> MSLRPLYMDVQATTPLDPRVLDAMLPYLINYYGNPHSRTHAYGWESEAAMERARQQVASLIGADPREIIFTSGATESNNIAIKGVARFYRSRKKHLITTQTEHKCVLDSCRSLEAEGFQVTYLPVQKSGIIDLKELEAAIQPDTSLVSVMTVNNEIGVKQPIAEIGRICSSRKVYFHTDAAQAVGKIPLDVNDMKIDLMSISGHKIYGPKGVGAIYIRRRPRVRVEALQSGGGQERGMRSGTVPTPLVVGLGAACEVAQQEMEYDHKRISKLSERLIQNIMKSLPDVVMNGDPKHHYPGCINLSFAYVEGESLLMALKDVALSSGSACTSASLEPSYVLRAIGTDEDLAHSSIRFGIGRFTTEEEVDYTVEKCIQHVKRLREMSPLWEMVQDGIDLKSIKWTQH;> MGSSHHHHHHGSPTTENLYFQGHNMAASSRAQVLALYRAMLRESKRFSAYNYRTYAVRRIRDAFRENKNVKDPVEIQTLVNKAKRDLGVIRRQVHIGQLYSTDKLIIENRDMPRT;> MSTIEERVKKIIGEQLGVKQEEVTNNASFVEDLGADSLDTVELVMALEEEFDTEIPDEEAEKITTVQAAIDYINGHQA;> MAYHKKVVDHYENPRNVGSLDKTSKNVGTGLVGAPACGDVMKLQIQVDEKGKIVDARFKTFGCGSAIASSSLATEWVKGKTVEEALTIKNTDIAKELCLPPVKLHCSMLAEDAIKAALADYKLKQEPKKGEAEKKLEHHHHHH

Maturation of iron-sulfur proteins in eukaryotes is initiated in mitochondria by the core iron-sulfur cluster assembly (ISC) complex, consisting of the cysteine desulfurase sub-complex NFS1-ISD11-ACP1, the scaffold protein ISCU2, the electron donor ferredoxin FDX2, and frataxin, a protein dysfunctional in Friedreich’s ataxia. The core ISC complex synthesizes [2Fe-2S] clusters de novo from Fe and a persulfide (SSH) bound at conserved cluster assembly site residues. High-resolution cryo-EM structures obtained from anaerobically prepared samples provide snapshots that both visualize different stages of persulfide transfer from Cys381NFS1 to Cys138ISCU2 and clarify the molecular role of frataxin in optimally positioning assembly site residues for fast sulfur transfer. FXN binding to generate the intermediate (Fe-NSIAUX)2 complex strongly increases the rate of persulfide transfer from NFS1 to ISCU2 (yielding (Fe-NIAUSX)2), implying a dedicated physiological role of FXN in this step, but FXN’s precise mechanistic function remains unclear.

Symmetry expansion and subsequent local 3D classification allowed separation of FXN-bound (77%) (Fe-NIAUX)2 and FXN-lacking (23%) (Fe-NIAU)2 states, which were locally refined to resolutions of 2.4 Å and 2.7 Å, respectively. The ISCU2-bound Fe ion was coordinated by residues Cys381NFS1, Asp71ISCU2, Cys95ISCU2, and likely a water (W1) molecule. Although persulfidation of NFS1 in the absence of FXN occurred quickly (see below), we did not observe density for a Cys381NFS1-bound persulfide at the ISCU2 assembly site. Active-site residue His137ISCU2, although oriented toward the ISCU2 assembly site, is too distant to coordinate the metal (His-Nε—Fe distance of 4.8 Å), distinguishing it from the X-ray structure of (Zn-NIAU)2. Similarly, Cys69ISCU2 and Cys138ISCU2 are too far for Fe coordination. The Fe-containing conformation raised the important functional question of which Cys residue of ISCU2 may serve as the sulfur acceptor from the Cys loop Cys381NFS1. The latter is closest to the sulfur atoms of Cys95ISCU2 (3.8 Å) and Cys69ISCU2 (4.3 Å), yet rather distant from Cys138ISCU2 (6.5 Å), which might suggest that Cys95ISCU2 or Cys69ISCU2 would be the most likely candidates for persulfide transfer from Cys381NFS1. Intriguingly, His137ISCU2, which is hydrogen-bonded to the water ligand of Fe between Cys381NFS1 and Cys138ISCU2, appears to prevent a closer approach of the two Cys residues and to hinder direct sulfur transfer. Therefore, either a substantial conformational change is needed to make Cys138ISCU2 available as a direct sulfur acceptor, or one of the other Cys residues may serve as the intermediate or even final sulfur acceptor. When compared to the Fe coordination in Fe-U, our (Fe-NIAU)2 cryo-EM structure showed Cys69ISCU2 being replaced by Cys381NFS1, and His137ISCU2 being exchanged for a water molecule.Here we structurally and biochemically characterise the DLP pair from Campylobacter jejuni. The respective proteins, here called Cj-DLP1 (84.5 kDa) and Cj-DLP2 (71.2 kDa), were cloned, expressed and purified. Both DLPs are monomeric in solution and form a stable heterotypic tetramer, termed Cj-DLP1/2tetramer, with 2:2 stoichiometry when mixed. The tetramer is dominated by a 2-fold symmetry where Cj-DLP2 with its symmetry mate (termed Cj-DLP2α and Cj-DLP2β) form a central back-to-back cis dimer flanked on each side by Cj-DLP1 (termed Cj-DLP1α and Cj-DLP1β). Combined with GTPase activity and lipid binding, we present a mechanism for how the tetramer tethers and bridges distantly opposing membranes.

Crystals of Cj-DLP1/2tetramer were obtained in the apo state and the structure solved. As observed in solution, the asymmetric unit of Cj-DLP1/2tetramer comprises a heterotypic tetramer in 2:2 ratio. Both Cj-DLP1 and Cj-DLP2 have a core DLP-like fold with GTPase, neck and trunk domains. The N-terminal 16 amino acids of Cj-DLP2 form helix 1 (Cj-DLP2H1), which inserts into a groove within Cj-DLP1AD. Here, Cj-DLP2H1 is partially clamped by Cj-DLP1 G-domain helix 18 and terminates in close proximity to Cj-DLP1 hinge 2, meaning it is ideally positioned to modulate Cj-DLP1 conformation upon binding. Connection between the Cj-DLP2H1/Cj-DLP1AD complex and the bulk of Cj-DLP2 is therefore via a 9 amino acid random coil linker only (termed Cj-DLP2linker). Such architecture suggests that Cj-DLP2linker represents a flexible tether in which Cj-DLP1α and Cj-DLP1β will be free to explore, in a mode akin to restricted Brownian motion, a spectrum of positions and orientations relative to the central Cj-DLP2 dimer. Hinge 1 acts as a fulcrum with the trunks of Cj-DLP1α and Cj-DLP1β assuming significantly different conformations relative to each other. Cj-DLP1α forms an open linear conformation, whereas the Cj-DLP1β trunk is rotated in plane ~125° towards the neck C-terminus. While the trunk orientation is likely determined by crystal geometry here, the conformational variability reflects the flexibility of the hinge 1 neck-trunk interface.

>[2x]MKELFQKIWQNELQFLNFDAKFQDKSKLDTAECAIILSVNKDNYERYFLLKEFQELCKKIDLRVDIFSMQNAQICILNLFKSGFISKQDLLKALKILEKISKNTEIFDFILQEKVQSIDQKALFQNDFKELNTINLELQKLSFDENLKSRLQKTLEKFQNLEFNIAITGVMNAGKSSLLNALLKEDFLGVSNIPETANLTVLSYGKSEEAKIYFWDKKEWQNILESSHFNADLKEFIDKLDKSVNIEDFIKDKPLIQNIALCELKNFSSAKNKISALIKKIEIKSHLEFLKNNISIVDTPGLDDVVVQREIVTNEYLRESDFLIHLMNASQSLTQKDADFLVHCLLNSRLSKFLIVLTKADLLSKKDLEEVIVYTKESLKSRLVDLDENLVEKIDFLCVSAKMASDFYKGLASKESLQKSGMQEFENYLFNELYAGEKSKIALRAYKKELHLELKNILSEYEMQNRLIKENKQGVSEENQKLLLELQKQNTLLKEAQDEISNSIAKLKNIDSGIDNLVLLLAKKLKERLIDEFKYLKNNAQKLNLSRILNIVDITTKDGINDILREIKFENIKKIEELKTNLSLKYDFLKDDFDNGFEGFKDGISKNIDSIFQSEKFALLRLKIEKLSNLKSDLYELETNLDTVIFDTFKEFKMSEILNSLNINGAFFEFLNDKLKHYEKNQKSKLESLEKVLQSLKNQDANILNSFEENLEKIEKLKQLEMGLLNADKLHH;>GSHMQINLLNDFIKAYENTYSVSFDDSFKGRIQELCKELNEPFMHASYALENELKELVFSLDKNVNIAIIGQFSSGKSSLLNLILGRDCLPTGVVPVTFKPTFLRYAKEYFLRVEFEDGSDIITNIEKLAFYTDQRNEVKQAKSLHIFAPIPLLEKITLVDTPGLNANENDTLTTLDELKNIHGAIWLSLIDNAGKKSEEDAIKANLELLGENSICVLNQKDKLSAEELDNVLNYAKSVFLKYFNELIAISCKEAKDEQSYEKSNFQSLLDFLTQLDTTVLKEKFVKRKILNLCEILEDENQLFVGIFDRLLNQFQSYEKHLLLAYENFLKEIEILNHQILEQLKSISERISSEIFASVKEKDAYFYKESKGFLKKDLYTRYDYKAPYISSDDAFLAMFYNSDVMSKEFKKIKNELYKSFEEIKMKLKDFINILEREILLFKAEFSNIQKDHIFQSDKNFSELRAFCNASDEYFLKDFKELLFKSILELDLFFEKLNLKAFTNYENATKLSLAFFSRKINESRVLYELDSSEFVLFYPKKSEIYERVLNELNVYEFETLLINKPILTKIAKNFLEQSQNLIQEKNKFLDLKKAELQKRRAQILNVRESIKEDHH[2x]>VIGRLRGIILEKQPPIVLLETGGVGYEVHMPMTCFYELPEAGQEAIVFTHFVVREDAQLLYGFNNKQERTLFKELIKTNGVGPKLALAILSGMSAQQFVNAVEREELGALVKLPGIGKK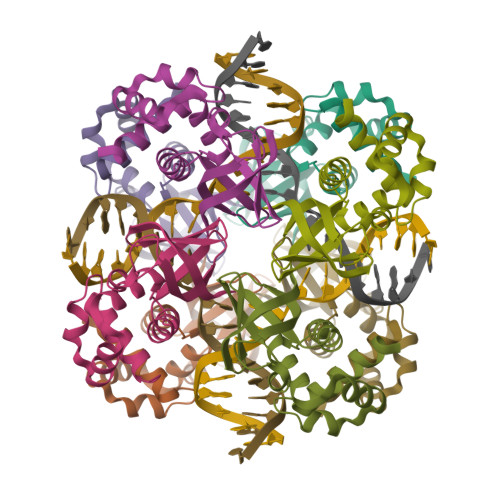TAERLIVEMKDRFK[8x]>MENSFKAALKAGRPQIGLWLGLSSSYSAELLAGAGFDWLLIDGEHAPNNVQTVLTQLQAIAPYPSQPVVAPSWNDPVQIKQLLDVGTQTLLVPMVQNADEAREAVRATRYPPAGIRGVGSALARASRWNRIPDYLQK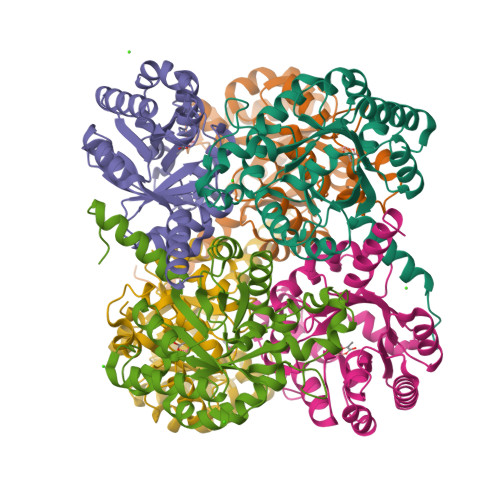ANDQMCVLVQIETREAMKNLPQILDVEGVDGVFIGPADLSADMGYAGNPQHPEVQAAIEQAIVQIRESGKAPGILIANEQLAKRYLELGALFVAVGVDTTLLARAAEALAARFGAQATA[6x]> GSMSEDIRRGPGRPPKKRVVPNFERKGILEKPVRPQSRLEFSYDNPLIFKNLFIYFKNLKSKNILVRCTPTEITFFSRDQSQASFVIATIDGKNVNHYYASDVFWLGINRELVEKMFNSIDRSFLKITIVHRYDKPETLFFIFTDFDIDKECTYQITVSEPELDMDLIEM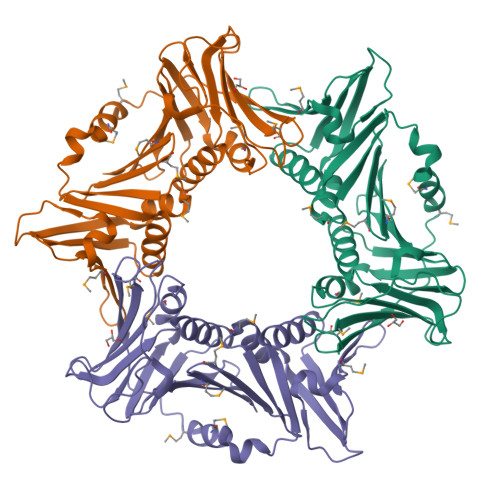EKSISEERLKNYPLRWEFTSKQLKKTFSDLSNYTELVTIEKLGGDTPLHLYFQKFNSISYHEMYKSSNKINLTSTIPKSQVFQINVKIAHIKSLASAMVTDKIRILCEENGNLIFQSEMDALMLNTITLNNTI>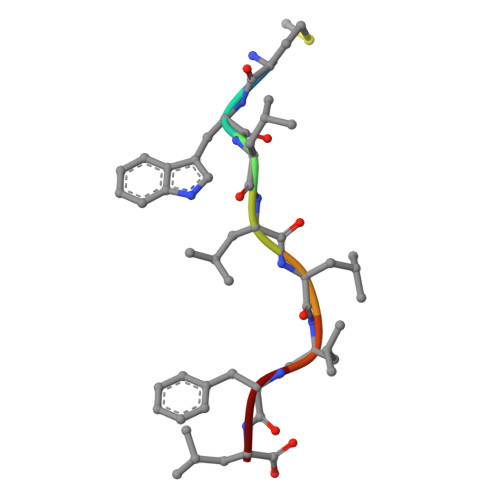 MWLLLLFL>GTQGKVIKCKAAIAWKTGSPLCIEEIEVSPPKACEVRIQVIATCVCPTDINATDPKKKALFPVVLGHECAGIVESVGPGVTNFKPGDKVIPFFAPQCKRCKLCLSPLTNLCGKLRNFKYPTIDQELMEDRTSRFTCKGRSIYHFMGVSSFSQYTVVSEANLARVDDEANLERVCLIGCGFSSGYGAAINTAKVTPGSTCAVFGLGCVGLSAIIGCKIAGASRIIAIDINGEKFPKAKALGATDCLNPRELDKPVQDVITELTAGGVDYSLDCAGTAQTLKAAVDCTVLGWGSCTVVGAKVDEMTIPTVDVILGRSINGTFFGGWKSVDSVPNLVSDY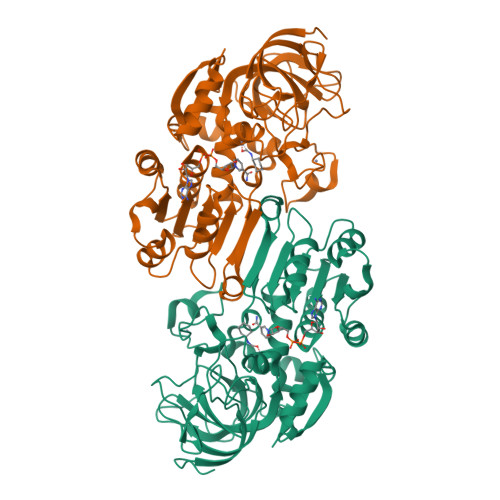KNKKFDLDLLVTHALPFESINDAIDLMKEGKSIRTILTF[2x]> GPHRSAAQMEVASFLLSKENQPENSQTPTKKEHQKAWALNLNGFDVEEAKILRLSGKPQNAPEGYQNRLKVLYSQKATPGSSRKTCRYIPSLPDRILDAPEIRNDYYLNLVDWSSGNVLAVALDNSVYLWSASSGDILQLLQMEQPGEYISSVAWIKEGNYLAVGTSSAEVQLWDVQQQKRLRNM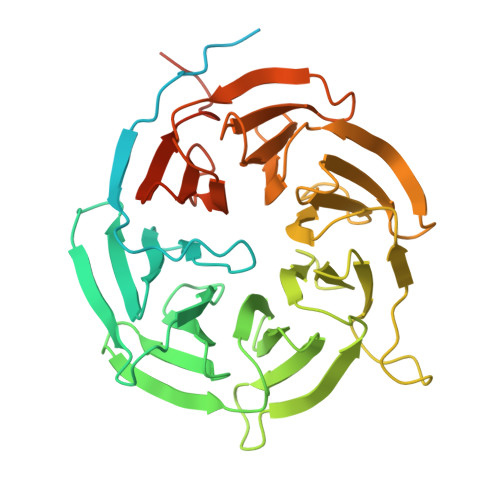TSHSARVGSLSWNSYILSSGSRSGHIHHHDVRVAEHHVATLSGHSQEVCGLRWAPDGRHLASGGNDNLVNVWPSAPGEGGWVPLQTFTQHQGAVKAVAWCPWQSNVLATGGGTSDRHIRIWNVCSGACLSAVDAHSQVCSILWSPHYKELISGHGFAQNQLVIWKYPTMAKVAELKGHTSRVLSLTMSPDGATVASAAADETLRLWRCFELDPARRREREKASAAKSSLIHQGIR>[4x]MGHHHHHHENLYFQMNTPTDLKVTKRDGRLEAIDLDKIHRVVTWAAEGLENVSVSQVELKSHIQFYNGIRTDDIHETIIKAAADLISEDTPDYQYLAARLAIFHLRKIAYGEYEPPHLYNHVKKLTDAGKYDRHILEDYSREEFDELNAYIDHERDMSFSYAAVKQLEGKYLVQNRVTRQIYETPQFLYVLVAMCLFSKYPKEARLDYVKRFYDAVSTFKVSLPTPIMSGVRTPTRQFSSCVLIECDDSLDSINATTSAIVKYVSQRAGIGINAGRIRGLDSEIRGGEARHTGCIPFFKMFQAAVKSCSQGGVRGGAATLFYPLWHIEAESLLVLKNNRGVEDNRIRQLDYGVQINRLLYTRLIKGGNITLFSPNEVSGLYEAFFADQDEFERLYTKYEQDPNIRKRIIPAADLFSTLMQERAGTGRIYIQNVDHCNTHSPFDPRVAPVHQSNLCMEIALPTKPLDNINDPDGEIALCTLSAFNLGALNSLDELEGLADLTVRALDALLDYQGYPVEAARTSTMDRRSLGIGVINYAYYLAKNGVRYSDGSALGLTHRTFEAIQYYLLKASANLAKEYGACTLFNQTVYSQGKLPIDTYKKDLDAVCGEPLHYDWESLRADIVKYGLRNSTLTALMPSETSSQIANATNGIEPPRGLVTVKASKDGILKQVVPEFETLKNAYETLWQLPGNEGYLKLVGVMQKFVDQAISANTAYDPGKFEGNKVSMKQMLKDLLTAYKYGVKTLYYHNTRDGADDTQTDIQDDGCAGGACKI;>MGHHHHHHENLYFQMSYSTFPKTKNDALKEPMFFGQPVNVARYDQQKYEVFEKLIEKQLSFFWRPEEIDVSRDRIDYANLPEHEKHIFISNLKYQTLLDSIQGRSPNVALLPLVSIPELETWVETWSFSETIHSRSYTHIIRNIVNDPSVVFDDIVENEYITARAEDIACYYDDLIEYTQYYNLLGEGVHNVGGKPVTVSLRGLKKKLY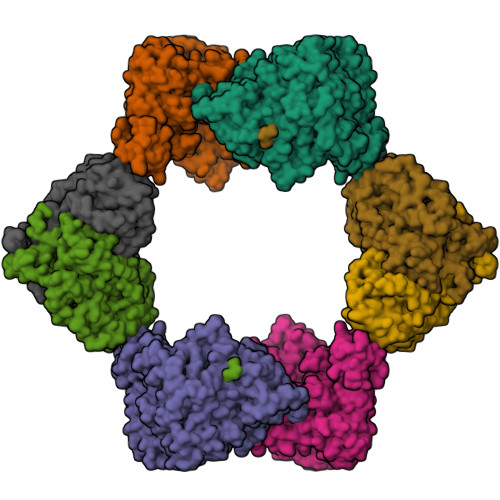LCLMCVNVLEAIRFYVSFACSFAFAERELMEGNAKIIKDIARDEALHLTGTQHMLNLMRSGVDDPEMAEIAAELQDECFQLFKKAAEQEKEWAAYLFKDGSMIGLNKEILSQYVEYITNLRMQAVGLPAGFEGANQNPIPWINAWLSSDNVQVAPQEVEISSYLIGQIDSEVNTDDLGDFEL[4x]> 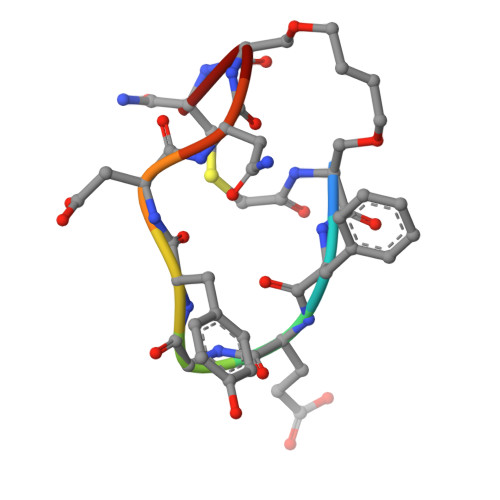SFEGYDNXC> GSHMAVQIGFLLFPEVQQLDLTGPHDVLASLPD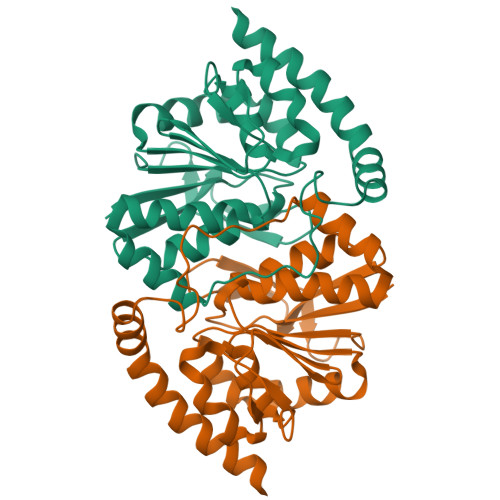VQVHLIWKEPGPVVASSGLVLQATTSFADCPPLDVICIPGGTGVGALMEDPQALAFIRQQAARARYVTSVCTGSLVLGAAGLLQGKRATTHWAYHELLAPLGAIPVHERVVRDGNLLTGTGITAGIDFALTLAAELFDAATAQRVQLQLEYAPAPPFNAGSPDTAPASVVQQARQRAADSLHKRREITLRAAARLAAG> MNAR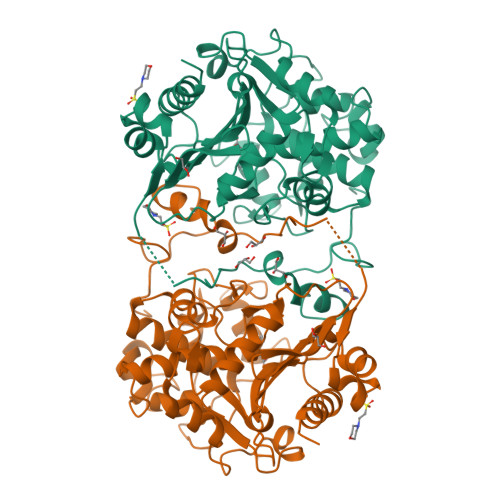STGQHPARYPGAAAGEPTLDSWQEPPHNRWAFAHLGEMVPSAAVSRRPVNAPGHALARLGAIAAQLPDLEQRLEQTYTDAFLVLRGTEVVAEYYRAGFAPDDRHLLMAVSKSLCGTVVGALVDEGRIDPAQPVTEYVPELAGSVYDGPSVLQVLDMQISIDYNEDYVDPASEVQTHDRSAGWRTRRHGDPADTYEFLTTLRGDGSTGEFQYCSANTDVLAWIVERVTGLRYVEALSTYLWAKLDADRDATITVDTTGFGFANGGVSCTARDLARVGRMMLDGGVAPGGRVVSEDWVRRVLAGGSHEAMTDKGFTNTFPDGSYTRQWWCTGNERGNVSGIGIHGQNLWLDPLTDSVIVKLSSWPDPDTEHWHRLQNGILLDVSRALDAV> MGKVRNISGCVAVAHGVRLAD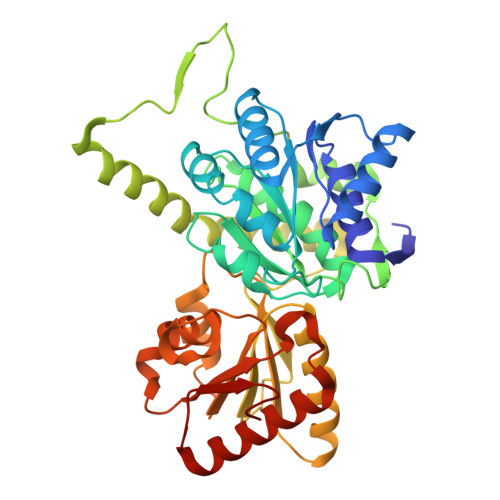VDVICSYPIRPYTGIMSELARMVADGELDAEFVHGEGEHAQLSVVYGASAAGARVFTGSSGVGVTYAMEVYSPISGERLPVQMAIADRTLDPPGDFGEEHTDAECCRDQGWIQGWASTPQEALDNTLIYYRVGEDQRVLLPQYACLDGYFVSHILGPVDIPDEAQVKEFLPPYKNHHVLDPRKPQIIGPQIEPAMGPPLQYQRYQAVKGVHKVLEEACDEFARIFGRKYDPYLDEYLTDDAEVIIFGQGAHMETAKAVARRLRNLGEKVGVARLRTFRPFPTEQIKERLSKFKAIGVLDVSANFGISCSGGVLLSELRAALYDYGDKVKTVGFVAGLGGEVVTHDEFYRMFQKLKEIAKTGKVEQTSYWIPFEL>SMLERTINLYPLTNYTFGTKEPLYEKDSSVAARFQRMREEFDKIGMRRTVEGVLIVHEHRLPHVLLLQLGTTFFKLPGGELNPGEDEVEGLKRLMTEILGRQDGVLQDWVIDDCIGNWWRPNFEPPQYPYIPAHITKPKE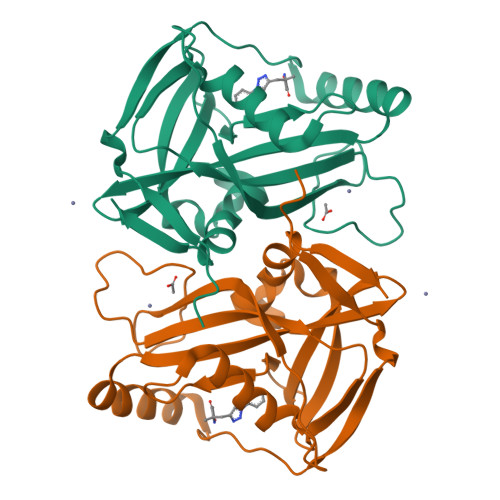HKKLFLVQLQEKALFAVPKNYKLVAAPLFELYDNAPGYGPIISSLPQLLSRFNFIYN[2x]> GAMGNNLVETTCKNTPNYQLCLKTLLSDKRSATGDITTLALIMVDAIKAKANQAAVTISKLRHSNPPAAWKGPLKNCAFSYKVILTASLPEAIEALTKGDPKFAEDGMVGSSGD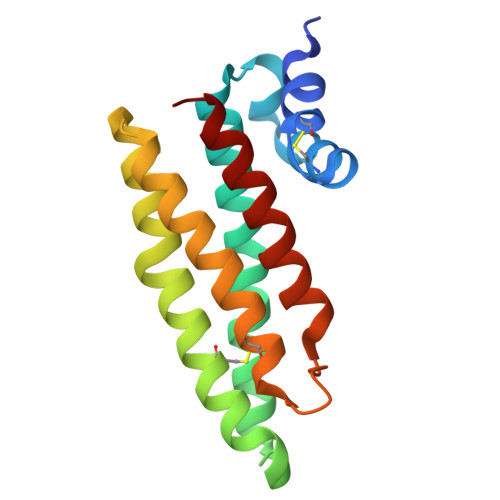AQECEEYFKGSKSPFSALNIAVHELSDVGRAIVRNLL>[2x]GAMEEKYLPELMAEKDSLDPSFTHALRLVNQEIEKFQKGEGKDEEKYIDVVINKNMKLGQKVLIPVKQFPKFNFVGKLLGPRGNSLKRLQEETLTKMSILGKGSMRDKAKEEELRKSG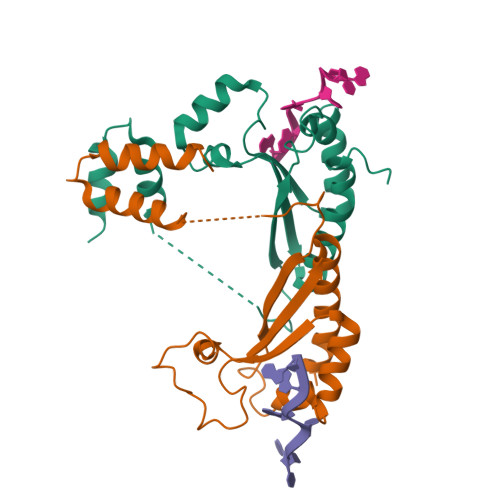EAKYFHLNDDLHVLIEVFAPPAEAYARMGHALEEIKKFLIPDYNDEIRQAQLQELTYLNGGSENADV4'-[7-(hydroxymethyl)-2,4-dihydroindeno[1,2-c]pyrazol-3-yl]biphenyl-4-ol 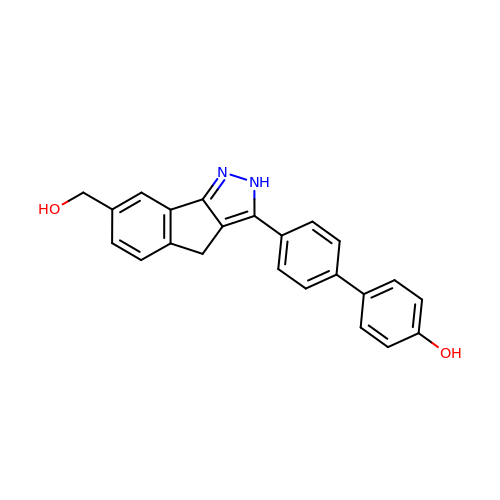| C23 H18 N2 O2 | BERKODPQGRAHDD-UHFFFAOYSA-N N-({(1R)-1-carboxy-2-[(4-fluorobenzyl)sulfanyl]ethyl}carbamoyl)-L-glutamic 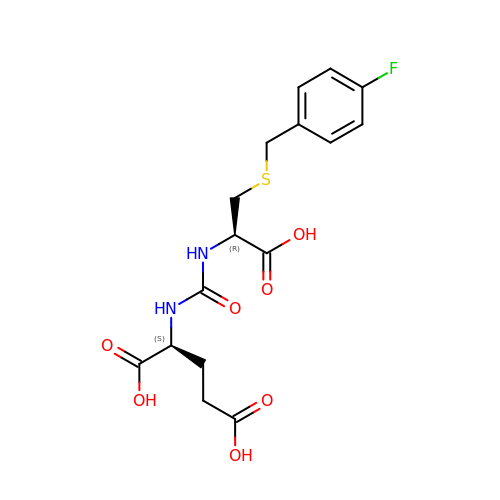acid | C16 H19 F N2 O7 S | IDTMSHGCAZPVLC-RYUDHWBXSA-N N-[(1R)-1-[3-(Cyclopentyloxy)-phenyl]-ethyl]-3-[(3,4-dihydro-2,4-dioxo-1(2H)-pyrimidinyl)methoxy]-1-propanesulfonamide | C21 H29 N3 O6 S 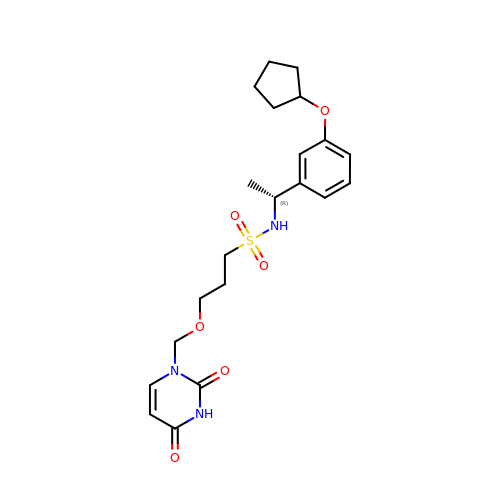| AMCGLRWKUQPNKD-MRXNPFEDSA-N>SNAERLAAWTRLPWEGLRYSYNRERRGTAARSCPQLEADVALKAETQPSEIPLERQLILEACREAERFGFLHELSIAI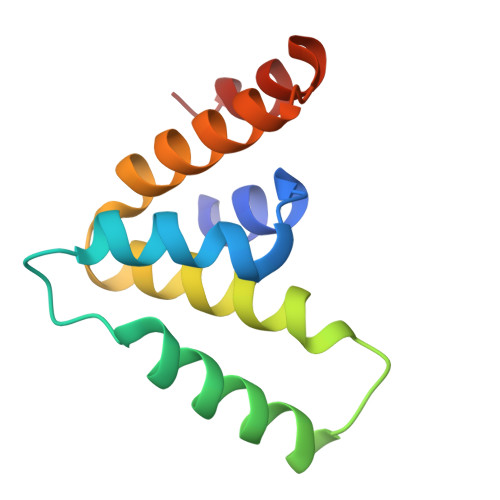VEMERLNKRPEAEVEEIAKLWQ[2x]>MLSRRYAAKSFVEWYYRQINENKPVASGYVNNNATYTKAGHPPADITINGRVVATPEEWDTMLKEQRAQHNTSSSSTLPIGRKPVRYDVDCFDVHVINADYRFAAPQRMIEQHAPTDGVRMMMALTVSGSVYFGASPRSTDDYVIKQHFNDVFILVPNWDVLEKPGARSGRKYLIASHKYRAY[2x]

The Mex67–Mtr2 complex (NXF1–NXT1 in metazoans and small bristles in Drosophila melanogastor) is the principal mRNA-export factor in Sacccharomyces cerevisiae. Mex67/NXF1 is a modular protein constructed from four domains: an RNA-recognition motif (RRM) domain, a leucine-rich repeat (LRR) domain, a nuclear transport factor 2-like (NTF2L) domain and an ubiquitin-associated (UBA) domain. Mtr2 is a ∼15–20 kDa protein that also has an NTF2-like fold and forms a tight heterodimeric complex with the Mex67 NTF2L domain.

In the complex, ctMtr2 was not altered when compared with the isolated structure, with a Cα r.m.s.d. of 0.38 Å over 148 residues. The UBA domains and Mtr2/NXT1 showed a high level of structural conservation (Cα r.m.s.d. < 0.8 Å), whereas the NTF2L domain showed the greatest variation (Cα r.m.s.d. = 1.9 Å).> MQPYWAAIEADIERYLKKSITIRPPETVFGPMHHLTFAAPATAASTLCLAACELVGGDRSQAMAAAAAIHLVHAAAYVHEHLPLTDG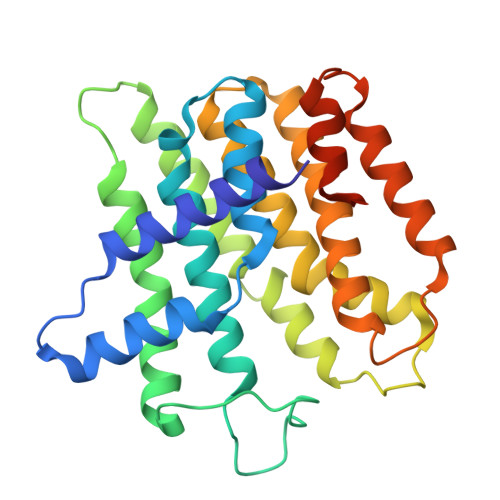SRPVSKPAIQHKYGPNVELLTGDGIVPFGFELLAGSVDPARTDDPDRILRVIIEISRAGGPEGMISGLHREEEIVDGNTSLDFIEYVCKKKYGEMHACGAACGAILGGAAEEEIQKLRNFGLYQGTLRGMMEMKNSHQLIDENIIGKLKELALEELGGFHGKNAELMSSLVAEPSLYAAHHHHHHHH>MKRMEGKLFMVSKKLQVVTKTVLLSTVFSISLLNNEVIKAEQLNINSQSKYTNLQNLKITDKVEDFKEDKEKAKEWGKEKEKEWKLTATEKGKMNNFLDNKNDIKTNYKEITFSMAGSFEDEIKDLKEIDKMFDKTNLSNSIITYKNVEPTTIGFNKSLTEGNTINSDAMAQFKEQFLDRDIKFDSYLDTHLTAQQVSSKERVILKVTVPSGKGSTTPTKAGVILNNSEYKMLIDNGYMVHVDKVSKVVKKGVECLQIEGTLKKSLDFKNDINAEAHSWGMKNYEEWAKDLTDSQREALDGYARQDYKEINNYLRNQGGSGNEKLDAQIKNISDALGKKPIP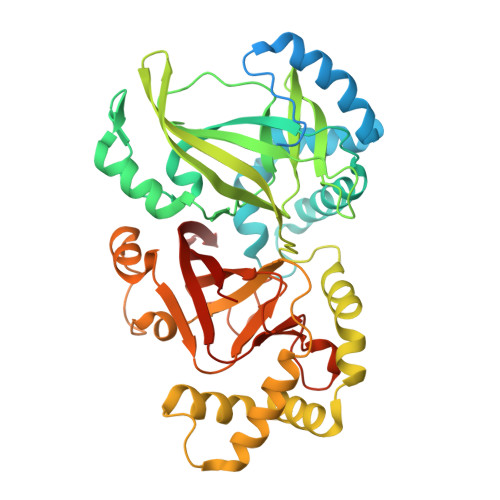ENITVYRWCGMPEFGYQISDPLPSLKDFEEQFLNTIKEDKGYMSTSLSSERLAAFGSRKIILRLQVPKGSTGAYLSAIGGFASEKEILLDKDSKYHIDKVTEVIIKGVKRYVVDATLLTN[4x]>[4x]MSALPPVYSFPPLYTRQPNSLTRRQQISTWIDIISQYCKTKKIWYMSVDGTVINDNELDSGSTDNDDSKKISKNLFNNEDIQRSVSQVFIDEIWSQMT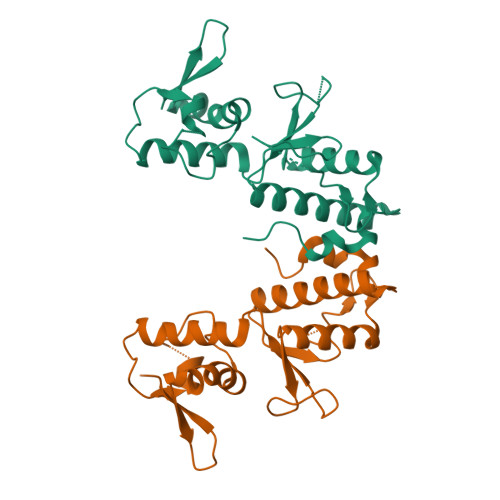KEGKCLPIDQSGRRSSNTTTTRYFILWKSLDSWASLILQWFEDSGKLNQVITLYELSEGDETVNWEFHRMPESLLYYCLKPLCDRNRATMLKDENDKVIAIKVV>[2x]ELWAKIANSINDINEQYLKVYEHAVSSYTQMYQDFSAVLSSLAGWISPGGNDGNSVKLQVNSLKKALEELKEKYKDKPLYPANNTVSQEQANKWLTELGG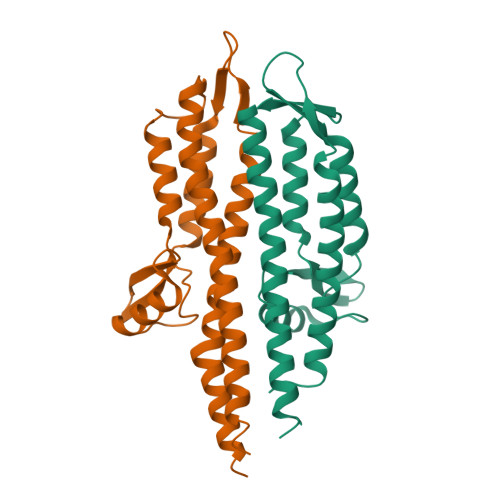TIGKVSQKNGGYVVSINMTPIDNMLKSLDNLGGNGEVVLDNAKYQAWNAGFSAEDETMKNNLQTLVQKYSNANSIFDNLVKVLSSTISSCTDTDKLFLHF>MSLKIAVLDDYQDAVRKLDCFSLLQDHEVKVFNNTVKGVGQLAARVADVEALVLIRERTRVTRQLLDRLPKLKIISQTGRVSRDAGGHIDLEACTDKGVVVLEGKGSPVAPAELTWALVMAAQRRIPQYVASLKHGAWQQSGLKSTTMPPNFGIGRVLKGQTLGIFGYGKIGQLVAGYGRAFGMNVLVWGRENSKERARADGFAVAESKDALFEQSDVLSVHLRLNDETRSIITVADLTRMKPTALFVNTSRAELVEENGMVTA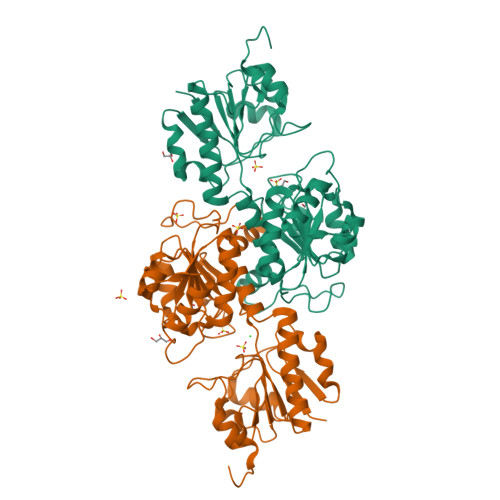LNRGRPGMAAIDVFETEPILQGHTLLRMENCICTPHIGYVERESYEMYFGIAFQNILDILQGNVDSVANPTALAPALIRAEGHHHHHH[4x]>[3x]EEGLDFPEYDGVDRVVNVNAKNYKNVFKKYEVLALLYHEPPEDDKASQRQFEMDELILELAAQVLEDKGVGFGMVDSEKDAAVAKKLGLTEEDSVYVFKGDEVIEYDGEFSADTLVEFLLDVLEDPVELIEGERELQAFENIEDDNKLIGYFKNKDSEHYKAYEDAAEEFHPYIPFFATFDSKVAKKLTLKLNEIDFYEAFMEEPVTIPDKPNSEEEIVSFVEAHKRSTLRKLKPESMYETWEDDLDGIHIVAFAEETDPDGYEFLETLKAVAQDNTDNPDLSIIWIDPDDFPLLVPYWEKTFNIDLSAPQIGVVNVTDADSVWMEMDDEEDLPSAEELEDWLEDVLEGEINTEDDDEEDD

Calsequestrin (Casq) is considered to be the major Ca2+-storage/buffer protein within the sarcoplasmic reticulum (SR) of both cardiac and skeletal muscle, where it resides as either its cardiac (Casq2) or skeletal (Casq1) isoform. Casq binds Ca2+ with a capacity roughly equivalent to a half of its total negative charge and an overall dissociation constant of ~1 mM. When studied in solution, Casq polymerizes as free Ca2+ concentrations increase and depolymerizes as Ca2+ concentrations decrease. We also showed that both glycosylation and phosphorylation alter the physical characteristics of Casq substantially, including its oligomerization and Ca2+-binding capacity.

Low-Ca2+ native bovine Casq1 crystallized in the P1 space group and contained four molecules in the unit cell; the resolution of its diffraction data was 2.74 Å, whereas low-Ca2+ recombinant bovine Casq1 crystallized in the C2221 space group and contained one molecule in the asymmetric unit, with a resolution of 1.88 Å. Both high-Ca2+ native and recombinant bovine Casq1 crystallized in the C2221 space group with three molecules in the asymmetric unit at resolutions of 2.60 and 2.14 Å, respectively. On the other hand, the three molecules in the high-Ca2+ asymmetric unit of native and recombinant corresponded to one-half of a linear hexamer. Residues 350 through 354 in the crystal structure of high-Ca2+ recombinant Casq1 could not be modeled because they were not resolvable, which indicates that residues 350 through 354 are inherently flexible. The larger structural variation among recombinant monomers, A, B and C, appeared to be due to a Leu246-mediated, Ca2+-dependent hydrophobic interaction that was only found in recombinant Casq1 upon exposure to a high Ca2+ concentration. Residues Glu244 through His250 normally form a loop stabilized by hydrogen bonds, a salt bridge (between Arg223 and Glu244) and hydrophobic interactions of Leu246 with nearby residues. In monomer B of the high-Ca2+ recombinant Casq1, however, this loop was deformed upon binding of one Ca2+ ion by the carboxylate sidechains of Asp245 and Asp247 and the backbone carbonyl group of Ile249. Consequently, the bound Ca2+ ion displaced the sidechain of Leu246 and swung it outward across the back-to-back interface and into a hydrophobic pocket formed by Ala20, Tyr23, Ala82 and Val83 of chain A. The Ca2+-dependent loop deformation also forced the backbone carbonyl of Gly248, which hydrogen bonds with the backbone amide of Val317 located in the middle of the N-linked glycosylation consensus sequence (316NVT318), downward against the glycosylation loop, which shifted the glycosylation loop accordingly. The net effect of the outward shift of α12 in monomer A and the Leu246-mediated, Ca2+-dependent hydrophobic interaction between monomers A and B was a break of the back-to-back symmetry.In M. capsulatus (Bath), two related β-sheet proteins (31% sequence identity) have been previously identified, a cytochrome P460 (McP460) and a cytochrome c′ (McCP-β)5,6 encoded by the CytL and CytS genes respectively. Cytochromes P460, defined by an unusual porphyrin-Lys cross link at the 13′ meso carbon, catalyse the oxidation of hydroxylamine (NH2OH) to form N2O under anaerobic conditions. In contrast, cyts cp-β (the only known cytochromes c′ with a β-sheet fold) lack this crosslink and appears to be optimized for binding non-polar molecules (including NO and CO) without enzymatic conversion. High resolution crystal structures reveal a highly similar tertiary structure between the two proteins but major structural differences around the heme pocket consistent with a switch of function between hydroxylamine oxidation (P460) and NO binding/sequestration (cyt cp-β).

The crystal structure of McCP-β was solved by SAD using the anomalous signal of the intrinsic heme Fe, and the structure determined to 1.61 Å resolution. McCP-β displays a highly β-sheet fold that is quite unlike any known cytochrome c′ structures (all previous examples being 4 α-helix bundles), yet very similar to McP460 (Fig. 1 and S3†). McCP-β exhibits a novel distal pocket structure relative to NeP460, McP460 and all cyt cp-α structures. The pocket is comprised of hydrophobic residues, with two aromatic Phe residues (Phe 32 and Phe 61) centrally located above the Fe in a ‘capping’ position well-suited to sterically influencing the binding of diatomic ligands (we name this structural feature the ‘Phe Cap’). In contrast to the structures of cyt P460, no heme-protein crosslink is observed in the McCP-β structure and the equivalent residue, Phe 61, now forms part of the Phe cap. In contrast to McP460, there is no porphyrin-Lys cross-link or potential H-bonding residue to interact with heme-bound water or diatomic ligands in McCP-β, and indeed the heme is 5-coordinate in the resting state with a vacant distal heme binding site. The proximal pocket contains the conserved haem ligand His 123 and an aromatic Phe 133 residue (oriented perpendicular to the imidazole plane), analogous to all reported cyt P460 structures this arrangement differs from that of cyts cp-α in which a conserved positive, polar residue (Arg or Lys) lies adjacent to the His ligand. The McCP-β structure also shows that the His ligand forms a H-bond to the carbonyl of Tyr 99, analogous to the situation in McP460. The heme pocket of McCP-β is much less solvent-exposed than in McP460 with a highly hydrophobic distal pocket with no water molecules observed within the McCP-β heme pocket. In the low frequency region, the ν(Fe–His) vibration of Fe(ii) McCP-β is evident at 219 cm–1, which is ∼10–15 cm–1 lower than for Fe(ii) cyt cp-α proteins, suggesting that McCP-β has a weaker proximal bond.

>[2x]MNKPSFLLVGLLVVSGVLGAAETKVKYPDGFRSWYHVKSMVIQPGHPLENPFGGIHHVYANAEAIQGLRGGNYPDGAVLVFDLFDYQEDNHALVEGKRKLIGVMERDAKRFSATGGWGYEGFGEGKPDKRLVTDGGQGCFGCHAAQKESQYVFSRLRD> TETTSFLITKFSPDQQNLIFQGDGYTTKEKLTLTKAVKNTVGRALYSSPIHIWDRETGNVANFVTSFTFVINAPNSYNVADGFTFFIAPVDT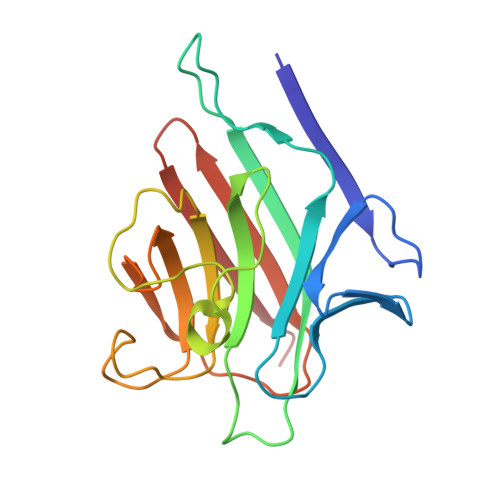KPQTGGGYLGVFNSAEYDKTTQTVAVEFDTFYNAAWDPSNRDRHIGIDVNSIKSVNTKSWKLQNGEEANVVIAFNAATNVLTVSLTYPN> SMIVRGINMTKIKLESPGFMVHKKLKSMSQSYGVMMTGVPAEVLGQMQAERSIPSINKTGNLKQQIAKEVSKVCHMMTEPTQSCGQASNDVC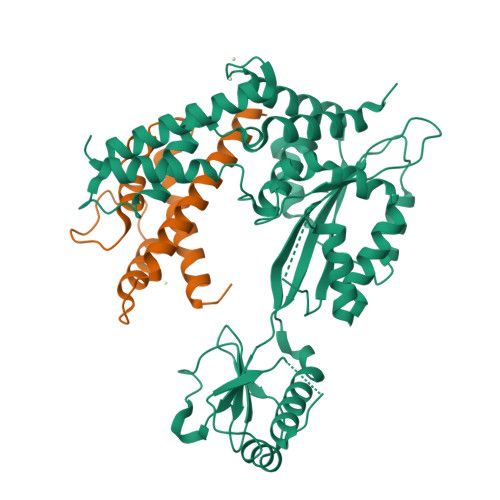ELLLGKIEAEKFHFTKYEALSADGDNLKNVLENTAPSSTNLLIRFEIDREDPPIVLVKTKNENFNPETAVKNKIYLLENKLYFIDKMGNLFNLGPGKKKCTQLFNAIGDSAEYSLCDPFVLEEPEKPEDFAISEIVDIFNEQKERFDFWIGSHSFTIYIPQTLGESPRQFYPYQAYFGSHTLQDWFVSDKDEYLSRIGIDKYIEKLAVLGKTTNTKERSDIYAEFFSKRGREAFFCAHLNEKRQPLRVKFKITEINPELALKNLQETQEFIDTHPGENPSDKVENYRNRAKLAMTEHLESLLDIKPESS;> SGTFFKDYQKKNVMRLLQDSLEKIINEWLKTDDESHTKLKSLQELSEMDINATSFAEHSPLPDFVTRLWLDPHKALDAMDKNISKNEIRKLIKETAREIELVFTHQK>[6x]MIPVTELRYFADTQPAYRILKPWWDVFTDYISIVMLMIAVFGGTLQVTQDKMICLPCKWVTKDSCNDSFRGWAASSPEPTYPNSTVLPTPDTGPTGIKYDLDRHQYNYVDAVCYENRLHWFAKYFPYLVLLHTLIFLACSNFWFKFPRTSSKLEHFVSILLKCFDSPWTTRALSETVVEESDPKPAFSKMNGSMDKKSSTVSEDVEATVPMLQRTKSRIEQGIVDRSETGVLDKKEGEQAKALFEKVKKFRTHVEEGDIVYRLYMRQTI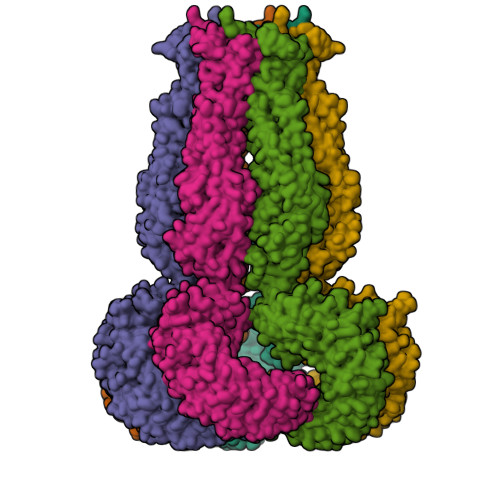IKVIKFALIICYTVYYVHNIKFDVDCTVDIESLTGYRTYRCAHPLATLFKILASFYISLVIFYGLICMYTLWWMLRRSLKKYSFESIREESSYSDIPDVKNDFAFMLHLIDQYDPLYSKRFAVFLSEVSENKLRQLNLNNEWTLDKLRQRLTKNAQDKLELHLFMLSGIPDTVFDLVELEVLKLELIPDVTIPPSIAQLTGLKELWLYHTAAKIEAPALAFLRENLRALHIKFTDIKEIPLWIYSLKTLEELHLTGNLSAENNRYIVIDGLRELKRLKVLRLKSNLSKLPQVVTDVGVHLQKLSINNEGTKLIVLNSLKKMVNLTELELIRCDLERIPHSIFSLHNLQEIDLKDNNLKTIEEIISFQHLHRLTCLKLWYNHIAYIPIQIGNLTNLERLYLNRNKIEKIPTQLFYCRKLRYLDLSHNNLTFLPADIGLLQNLQNLAVTANRIEALPPELFQCRKLRALHLGNNVLQSLPSRVGELTNLTQIELRGNRLECLPVELGECPLLKRSGLVVEEDLFSTLPPEVKERLWRADKEQA>VTLDGGAVAAPDQYGAKVAAEILKKGGNAVDAAVATAFTLAVTYPEAGNIGGGGFMTLYVDGKPYFLDYREIAPKAATKTMYLNEKGEVIENLSLVGAKAAGVPGTVMGLWEAHQRFGKLKWSELLTPAIGYAQTGFKVADQQYQYRQDAIALFNGKTNFGDYFGTMKPGEVFKQPELAKTLERIADKGPDDFYKGETAKLLIAQMKQDGGLITSDDLVDYQAKWREPMRIDWQGNTLYTAPLPSSGGIALAQLIGIKEQRAADFKGVELNSAKYIHLLSEIEKRVFADRADYLGDPQFSKVPVAQLTDPKYIAKRAGEVNPDAISATEKVRPGLEPHQ[2x];>[2x]TTHFSIVDKDGNAVSNTYTLNWDFGSGVVVKGAGFLLNDEMDDFSSKPGVANAFGVVGSDANAIEPGKRMLSSMSPSIVTR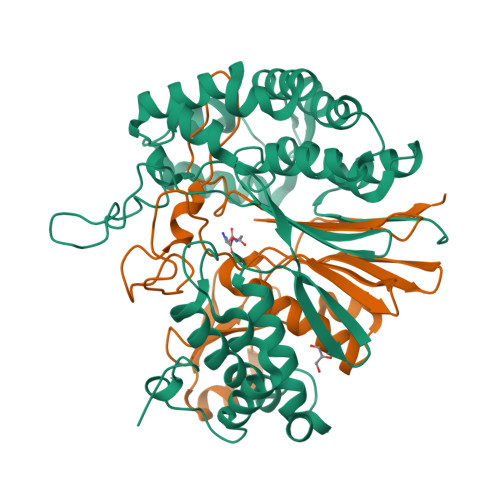DGHVSLVLGTPGGSRIFTSIFQVLNNVYDFHLPLEKAVAAQRVHHQLLPKDTIYYDAYAPLTGKVADELKAMGYTLEDQGWNMGDIQAIRVNGKALETASDPRGRGVGMVVKP> MVLRKVVAILLAILPIFLFAVEPIKVVRSEKEIVVLTRFEEYHFDLEKGILKDFYTLVDGRKHVFTYGNDGFDVLDEGTPLTVIEEPIVTGVGKVSEGFSDEVSIVYNYGYVKKIFTIKNNENYTFFVDIENSKPVDVTVPRVSVDTSTDRYLENYFASFNPKTRTLVLLKHDEGLLFEGTLKVNGQKRFIVFMGPNKRTLIKKAFPEDY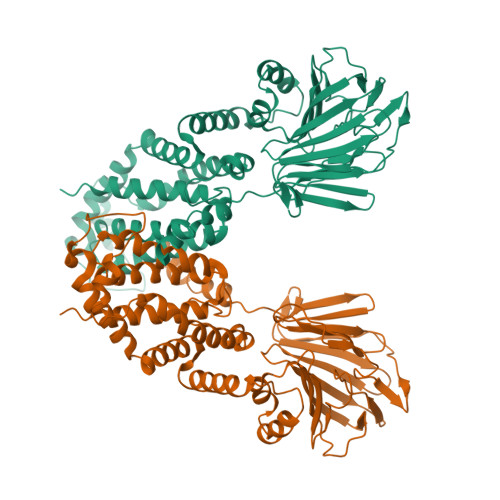DVLIKALVNIPGFNKWYDSVFYGLVWFFWWLKDLTKNFGWAIMLFTLIVRLILYPLYHAQTKSLINMRKLQPQIEAIKKKYKDPTKQQEALLKLYREAGVNPASGCLMLLIQLPIFMLLWSVIRYYVEEFAYSGSFLIWKDLSAGGFSNNWLFLVITIVASYYTTLLTSQDARTAWQGIIMSVIFPFLFVGLPSGLFLYYATNTLIQLAVTYYTY> FDLDDVQPNKAVEPEKTKVNYTDEETQKRKKEELDKLMEPALGYVTKIPVNIPSVRKTEISEIDTVTDESLSLVPNEDKLRTIANENYGSVVTKSGSNTMNFVRSGYTIDVVHYGLRDKGYVYYKGVHPSKELPKGNIIVYQGEWDFTSNADLDAKRPNYNPEFNGYGAGQRVGVTSADAKERTYISKFNIDFSNKKLNGQLLTKTKENQEKLRYTVEANISGNRFRGKATATDKTDPILGKDSEHLEGGLYGPKSEELAGKFVAHDKSLFAVFSGKRGNDVLETVKIIDASKIDLTTFESSELNNFGNANVLIIDGQKIDLAGADFKNRKTVDINGKTMVAIACCSNLEYMKFGQLWQKEGEQTKDNSLFLQGERTATDKIPVGGNYK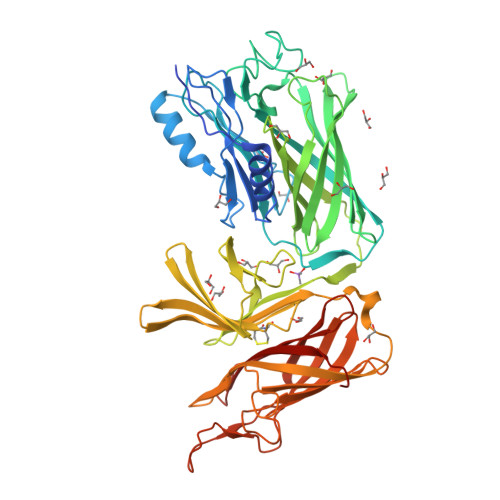YVGTWDALVSKGTNWVAEADNNRESGYRSEFDVNFGDKKVSGKLFDKGGIVPVFMINADIKGNGFTGTANTTDTGFALDSGSSQHGNAVFSDIKVNGGFYGPTAGELGGQFHHKSDNGSVGAVFGAKRQIEK>PKKQTRLGLEAKKEENLADWYSQVITKSEMIEYHDISGCYILRPWAYAIWEAIKDFFDAEIKKLGVENCYFPMFVSQSALEKEKTHVADFAPEVAWVTRSGKTELAEPIAIRPTSETVMYPAYAKWVQSHRDLPIKLNQWCNVVRWEFKHPQPFLRTREFLWQEGHSAFATMEEAAEEVLQILDLYAQVYEELLAIPVVKGRKTEKEKFAGGDYTTTIEAFISASGRAIQGGTSHHLGQNFSKMFEIVFEDPKIPGEKQFAYQNSWGLTTRTIGVMTMVHGDNMGLVLPPRVACVQVVIIPCGITNALSEEDKEALIAKCNDYRRRLLSVNIRVRADLRDNYSPGWKFNHWELKGVPIRLEVGPRDMKSCQFVAVRRDTGEKLTVAENEAETKLQAILEDIQVTLFTRASEDLKTHMVVANTMEDFQKILDSGKIVQIPFCGEIDCEDWIKKTTARDQDLEPGAPSMGAKSLCIPFKPLCELQPGAKCVCGKNPAKYYTLFGRSY[2x]

Aminoacyl-tRNA synthetases (aaRSs) are an essential enzyme family for protein translation and, in several cases, have been validated drug targets. Among the aaRSs, prolyl-tRNA synthetase (PRS) is a validated drug target in Plasmodial spp and Toxoplasma gondii (Tg). In the current study, we examined five ATP-mimetics L95, L96, L97, L35, and L36, based on the 1-(pyridin-4-yl) pyrrolidin-2-one (PPL) scaffold. We successfully co-crystallized all five compounds with TgPRS (L95, L96, L97, L35, and L36) and three with HsPRS (L95, L96, and L97), all in complex with L-pro.

The complex structure of HsPRS with L95, L96, and L97 was determined to address the structural basis for differential inhibition. The loop 1152–1165 exhibited ligand-induced fitting, and the residues Arg1152, Trp1153, Phe1155, Lys1156, and Arg1163 formed a cavity-like structure to fit L95, L96, and L97. However, three out of five PPL derivatives, i.e., L97, L96, and L35, were found to be selective against TgPRS as opposed to its human counterpart in vitro, with enzymatic selectivity indices of 27.9, 13.5, and 8.2, respectively. Based on the TgPRS enzyme data, L97 showed the highest selectivity index of 27.9 compared with the other four PPL derivatives. Structurally, in both TgPRS and HsPRS complex, L97 shared conserved interaction points except the H-bond between the O atom of hydroxymethyl attached to the pyrrolidine group with OG1 of Thr558, which is missing in HsPRS. This is due to a slight displacement of the hydroxyl group and, in turn, a slight downward displacement of the entire cyclopropyl-oxo-pyrrolidine group, sufficient enough to overcome the hydrophobic environment resulting from the exposed cyclopropyl core. In addition, the guanidinium moiety of Arg1163 is slightly displaced away from the pyrazole ring to form an H-bond with the OE1 atom of neighboring Gln1159 resulting in loose stacking of the entire 4-(3-Fluorophenyl)-1-methylpyrazole moiety in the ATP pocket. This is also evident in the rotameric conformations in Lys1156 and Phe1155.> MDRKLDEFIGDATPKKVSKEKPVRRKKRLKPTSLDSFLPEEHINYFRDLRIGSKKIRNA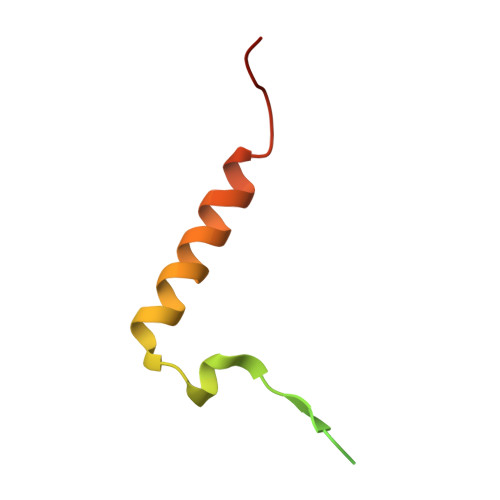KIEEL The first structure of the catalytic domain of RpfC (Rv1884), one of the resuscitation-promoting factors (RPFs) from Mycobacterium tuberculosis, is reported. Resuscitation-promoting factors (RPFs) have attracted much interest since their discovery in the late 1990s. These proteins resuscitate bacteria that have entered a dormant state, allowing them to proliferate normally. Later, various experiments unambiguously demonstrated that the RPF domain is a peptidoglycan hydrolase. The mycobacterial RPF proteins share a common 70-amino-acid RPF domain and the presence of N-terminal signal sequences suggesting that the proteins are translocated to an extracellular location.

The structure was solved using molecular replacement once the space group had been correctly identified as twinned P21 rather than the apparent C2221 by searching for anomalous scattering sites in P1. The asymmetric unit consists of eight copies of the RpfC chain. Chains A, E and S have the most residues modelled into electron density (Gly1–Lys86) with an extra helix beyond the end of the conserved domain (Gly78). Chain B has the least modelled residues (Pro4–Gly78); the other chains are between these limits. The final refined twinning fraction in REFMAC5 for the deposited structure was 0.463 for . Despite soaking and co-crystallizing with a range of substrates and substrate fragments, for example N-acetyl­glucosamine (NAG), polymers of up to five repeats of N-acetylglucosamine and NAG-N-acetylmuramic acid, and peptido­glycan fragments that are generated by a number of enzymes, we never obtained clear density for substrates in the active site. The structure displays a very high degree of structural conservation with the previously published structures of the catalytic domains of RpfB (Rv1009) and RpfE (Rv2450). In RpfC two residues display an elongated conformation (42GVGN45), very similar to RpfE (137GSGS140), to connect α-helices 2 and 3, while a 310-helix (321GLRYAPR327) is present in RpfB. Based on the structure that we have solved, we propose that the five RPFs from M. tuberculosis have similar substrates, although variation in charge around the active site may give rise to small variations in the specificity for different peptidoglycan modifications. The high degree of conservation of the RPF domain explains why the protein is functionally redundant, but most importantly shows that the auxiliary domain composition is mainly responsible for the functional variability.

>[8x]GPSPNWDAVAQCESGGNWAANTGNGKYGGLQFKPATWAAFGGVGNPAAASREQQIAVANRVLAEQGLDAWPTCGAASGLPIALWSKPAQGIK> EHIPP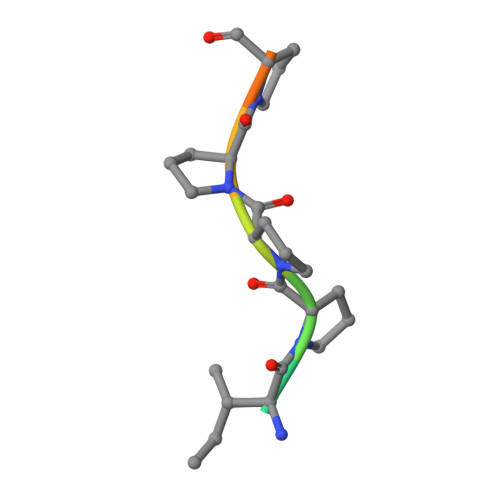PPRPP>QPRPAFSAIRRNPPMGGNVVIFDTVITNQEEPYQNHSGRFVCTVPGYYYFTFQVLSQWEICLSIVSSSRGQVRRSLGFCDTTNKGLFQVVSGGMVLQLQQGDQVWVEKDPKKGHIYQGSEADSVFSGFLIFPSA[2x];>ATQKIAFSATRTINVPLRRDQTIRFDHVITNMNNNYEPRSGKFTCKVPGLYYFTYHASSRGNLCVNLMRGRERAQKVVTFCDYAYNTFQVTTGGMVLKLEQGENVFLQATDKNSLLGMEGANSIFSGFLLFPDMEA[2x];>[2x]KQKFQSV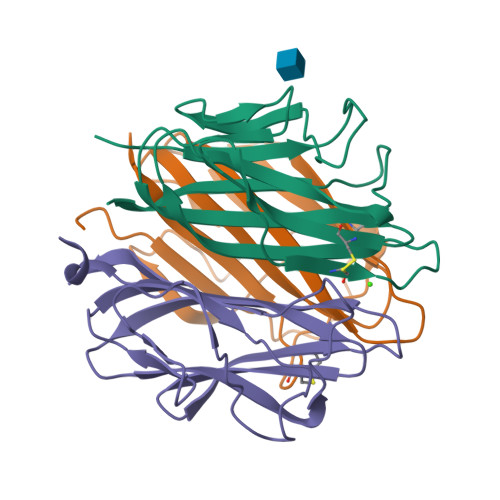FTVTRQTHQPPAPNSLIRFNAVLTNPQGDYDTSTGKFTCKVPGLYYFVYHASHTANLCVLLYRSGVKVVTFCGHTSKTNQVNSGGVLLRLQVGEEVWLAVNDYYDMVGIQGSDSVFSGFLLFPD>[2x]SATIVNTTDDNFQ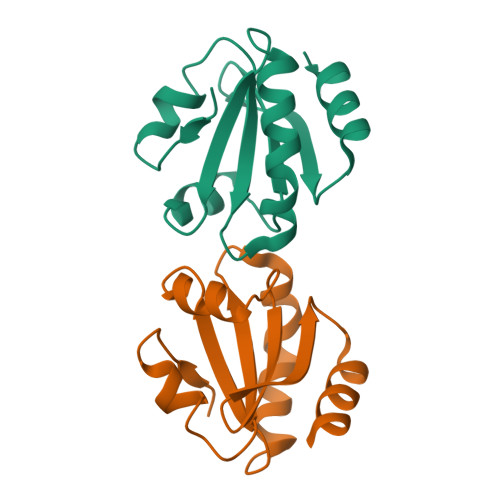ADVLDAETPVLVDFWAGWCAPCKAIAPVLEDLSSEYAGKVKIVKVDVTSCEETAVKYNIRNIPALLLFKNGEVVAQQIGAVPRSKLVSFIDENV>[6x]MADADPDVLKVALLPDENASELIKRNQPLKDYLEEHLDKKVQLIVTTDYSSMIEAMRFGRIDLAYFGPLSYVMAKSKSDIEPFAAMVIDGKPTYRSVIIANVASGVNEYADLKGKRMAYGDRASTSSHLIPKTVLLETADLTGGQDYEQHFVGTHDAVAVNVANGNADAGGLSEVIFNHAAERGLIDPSKVKVLGYSGEYPQYPWAMRSNLSPELKTKVRDVFVGIDDPEVLRNFKAEAFAPITDADYDVIRNMGSLLGLDFATMLEHHHHHH

Here we elucidate the molecular basis of high-affinity phosphite and hypophosphite acquisition by determining the ligand-binding affinity and structure of the PBPs of phosphite and hypophosphite ABC transporters from environmental microorganisms. We over-produced and purified PBPs of three putative phosphite transporters; PtxB from the globally important marine diazotroph Trichodesmium erythraeum IMS101 (Te_PtxB), PhnD from the oceanic picocyanobacteria Prochlorococcus marinus MIT9301 (Pm_PhnD)35 and PtxB from the soil bacterium Pseudomonas stutzeri WM88 (Ps_PtxB), as well as a PBP from a putative hypophosphite transporter, HtxB, also from P. stutzeri WM88 (HtxB)18. The structures reveal that ligand specificity, measured here by thermophoresis, arises from a combination of steric considerations and the interaction between a ligand P-H hydrogen atom and an aromatic π system in the binding pocket. The structures of two distinct types of phosphite-binding protein and a hypophosphite-binding protein reveal that a P-H…π interaction ensures high-affinity binding of specific ligands, representing a universal mechanism in these PBPs for recognising ligands with a P-H bond.

In our study, numerous attempts to crystallise apo forms of Te_PtxB and Pm_PhnD were unsuccessful, but a 2.1 Å resolution structure of Pseudomonas stutuzi PtxB (Ps_PtxB) in an open conformation was determined. Analysis of the conformational change between the open and closed, phosphite-bound structure of Ps_PtxB using DynDom42 revealed that domain closure is induced by a ~60° rotation around an axis that lies between the two lobes. This is facilitated by flexible loops that form the hinge region between the lobes (residues A85-T93 and Y200-Q202), as well as residues from the extreme end of the C-terminal helix (G255-L258). Superposition of the individual lobes of Ps_PtxB in the open and closed conformations shows that lobe 2 (residues 96–196, 0.35 Å RMSD cα) adopts a very similar structure, with the conserved STS-H motif (S124, T125, S126 and H155) spatially conserved in both conformations. In contrast, lobe 1 (residues 1–84 and 202–255, 1.55 Å RMSD cα) shows some differences between the open and ligand-bound states. The positions of Y94, which hydrogen bonds to one of the phosphite oxygen atoms in the closed structure, and D16, which hydrogen bonds to and stabilises the capping tyrosine in the closed structure, move ~7 Å and ~4.5 Å (cα-cα), respectively, on ligand binding. Y94 resides on the hinge region, the conformation of which alters substantially during domain closure, whilst D16 sits on a flexible loop that latches over the binding pocket in the closed conformation. In addition, the B-factors of the core residues in lobe 2 are much lower in the closed, ligand bound, conformation compared to those in the open structure, implying lower overall flexibility when phosphite is bound to the protein.> AVSLDRTRAVFDGSEKSMTLDISNDNKQLPYLAQAWIENENQEKIITGPVIATPPVQRLEPGAKSM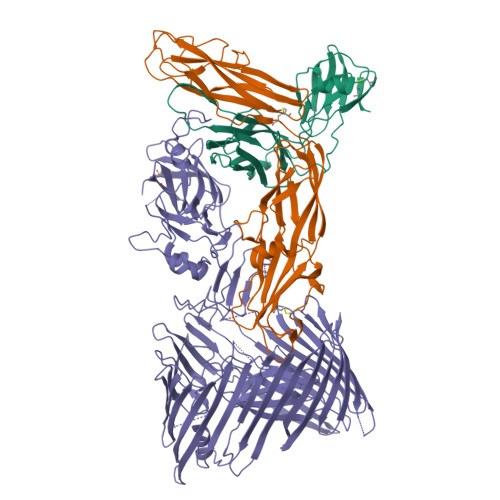VRLSTTPDISKLPQDRESLFYFNLREIPPRSEKANVLQIALQTKIKLFYRPAAIKTRPNEVWQDQLILNKVSGGYRIENPTPYYVTVIGLGGSEKQAEEGEFETVMLSPRSEQTVKSANYNTPYLSYINDYGGRPVLSFICNGSRCSVKHHHHHH;> WNNIVFYSLGDVNSYQGGNVVITQRPQFITSWRPGIATVTWNQCNGPEFADGFWAYYREYIAWVVFPKKVMTQNGYPLFIEVHNKGSWSEENTGDNDSYFFLKGYKWDERAFDAGNLCQKPGEITRLTEKFDDIIFKVALPADLPLGDYSVKIPYTSGMQRHFASYLGARFKIPYNVAKTLPRENEMLFLFKNIGGCRPSAQSLEIKHGDLSINSANNHYAAQTLSVSCDVPANIRFMLLRNTTPTYSHGKKFSVGLGHGWDSIVSVNGVDTGETTMRWYKAGTQNLTIGSRLYGESSKIQPGVLSGSATLLMILP;> VEFNTDVLDAADKKNIDFTRFSEAGYVLPGXXXXXXXXXXXXXXXXXXXXXXXXXXXXXXXXXXXXXXXXXXXXXXXXXXXXXXXXXXXXXXXXXXXXXXXXXXXXXXXXXXXXXXXXXXXLPPSRWDDGIPGLMLDYNLNGTVSRNYQGGDSHQFSYNGTVGGNLGPWRLRADYQGSQEQSRYNGEKTTNRNFTWSRFYLFRAIPRWRANLTLGENNINSDIFRSWSYTGASLESDDRMLPPRLRGYAPQITGIAETNARVVVSQQGRVLYDSMVPAGPFSIQDLDSSVRGRLDVEVIEQNGRKKTFQVDTASVPYLTRPGQVRYKLVSGRSRGYGHETEGPVFATGEASWGLSNQWSLYGGAVLAGDYNALAAGAGWDLGVPGTLSADITQSVARIEGERTFQGKSWRLSYSKRFDNADADITFAGYRFSERNYMTMEQYLNARYRNDYSSREKEMYTVTLNKNVADWNTSFNLQYSRQTYWDIRKTDYYTVSVNRYFNVFGLQGVAVGLSASRSKYLGRDNDSAYLRISVPLGTGTASYSGSMSNDRYVNMAGYTDTFNDGLDSYSLNAGLNSGGGLTSQRQINAYYSHRSPLANLSANIASLQKGYTSFGVSASGGAXXXXXXXXXXXXXXXXXXXXXXXXXXXXXXXXXXXXXXXXXXGKRLFAILRLADGSQPPFGASVTSEKGRELGMVADEGLAWLSGVTPGETLSVNWDGKIQCQVNVPETAISDQQLLLPCTPQKLVPRGSHHHHHH>MRGSHHHHHHGMASMRILLSNDDGVHAPGIQTLAKALREFADVQVVAPDRNRSGASNSLTLESSLRTFTFDNGDIAVQMGTPTDCVYLGVNALMRPRPDIVVSGINAGPNLGDDVIYSGTVAAAMA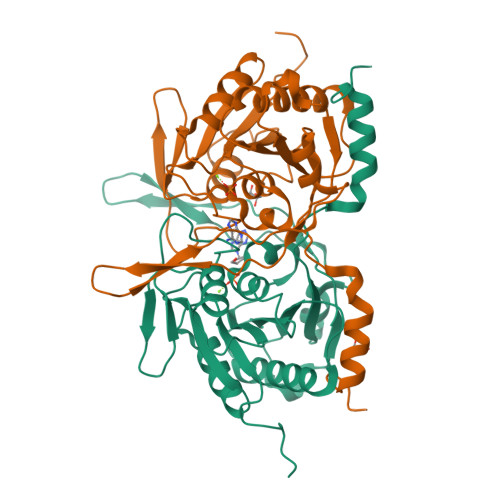GRHLGFPALAVSLNGYQHYDTAAAVTCALLRGLSREPLRTGRILNVNVPDLPLAQVKGIRVTRCGSRHPADKVIPQEDPRGNTLYWIGPPGDKYDAGPDTDFAAVDEGYVSVTPLHVDLTAHSAHDVVSDWLDSVGVGTQW[4x]>MGSHHHHHHENLYFQGHMNSFYSQEELKKIGFLSVGKNVLISKKASIYNPGVISIGNNVRIDDFCILSGKVTIGSYSHIAAYTALYGGEVGIEMYDFANIASRTIVYAAIDDFSGNALMGPTIPNQYKNVKTGKVILKKHVII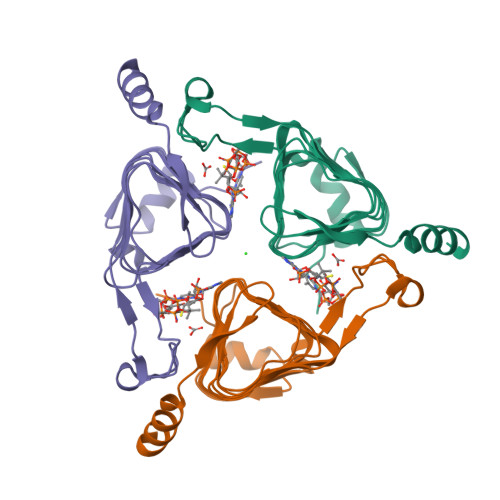GAHSIIFPNVVIGEGVAVGAMSMVKESLDDWYIYVGVPVRKIKARKRKIVELENEFLKSMNS[3x]We examined the crystal-packing interactions formed by the polo-box domain (PBD) of polo-like kinase 1 (Plk1), a validated anti-cancer target, whose phosphorylation-dependent protein–protein interactions are crucial for successful progression of the cell through mitosis. We have observed an unreported binding site in a number of crystal structures of the PBD, which is formed by the rearrangement of surface residues involved in crystal packing. This site is located close to the phosphopeptide-binding groove, making it potentially accessible for phosphorylated proteins binding to the PBD. The new binding site consists of seven residues: Val415, Leu478, and Phe482 form the bottom of the pocket whilst Tyr417, Tyr421, Tyr481, and Tyr485 form the sides of the pocket.

PBIP1 is involved in the localization of Plk1 to the kinetochores and its phosphorylation-dependent interaction with the PBD involving pThr78PBIP1 has been characterized. Only the PBIP1-derived peptide showed significant difference in thermal shifts for the wild-type (14.4 °C) and mutant protein (10.1 °C), so we decided to concentrate our efforts on this. The thermal shifts of 9.7 °C observed for 72-DPPLHSpTA-79 (lacking Phe71), and 10.5 °C observed for 71-ADPPLHSpTA-79 were significantly lower than the one observed for 71-FDPPLHSpTA-79 and showed no significant difference between the wild-type and mutant protein. Our thermal stability studies were further supported by isothermal titration calorimetry (ITC) measurements, which showed an increased affinity for the Phe71-bearing peptide. However, in the structure of the 71-FDPPLHSpTA-79–PBD complex, Phe71PBIP1 is found in the hydrophobic pocket. The side chain of Tyr481PBD rotates away from the domain to open the pocket, and the space between Tyr417PBD and Tyr485PBD is filled by Pro73PBIP1, closing the pocket around the side chain of Phe71PBIP1. The positions of Phe71PBIP1 and Pro73PBIP1 within the pocket are very similar to those observed previously for Phe8term and Pro6term in the crystal contact, despite the reversed direction of the peptide chain. Linker residues Asp72PBIP1 and Glu7term also adopt similar solvent-exposed conformations, but only the side chain of Asp72PBIP1 is ordered; the backbone nitrogen atom of this residue forms a hydrogen bond with the hydroxy group of Tyr417PBD.

>GPLGSPEFDCHLSDMLQQLHSVNASKPSERGLVRQEEAEDPACIPIFWVSKWVDYSDKYGLGYQLCDNSVGVLFNDSTRLILYNDGDSLQYIERDGTESYLTVSSHPNSLMKKITLLKYFRNYMSEHLLKAGANITPREGDELARLPYLRTWFRTRSAIILHLSNGSVQINFFQDHTKLILCPLMAAVTYIDEKRDFRTYRLSLLEEYGCCKELASRLRYARTMVDKLLSSR[3x];>XFDPPLHSTAX[3x]>MGGSHHHHHHLESTSLYKKSSSTPPRGVTVVNNFDCKRYLGTWYEIARFDHRFERGLEKVTATYSLRDDGGLNVINKGYNPDRGMWQQSEGKAYFTGAPTRAALKVSFFGPFYGGYNVIALDREYRHALVCGPDRDYLWINSRTPTISDEVKQEMLAVATREGFDVSKFIWV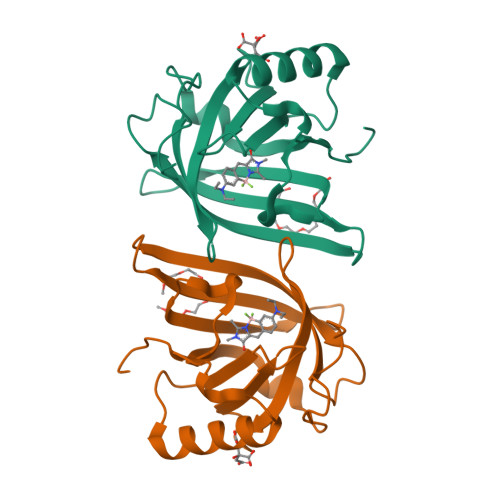QQPGS[2x]> QGFSLAQYLQEQKTIVETALDQSLVITEPVTIYEAMRYSLLAGGKRLRPILCLAACEMLGGTAAMAMNTACALEMIHTMSLIHDDLPAMDNDDLRRGKPTNHKVYGEDIAILAGDALLSYAFEYVARTPDVPAERLLQVIVRLGQAVGAEGLVGGQVVDLESEGKDVAVETLNFIHTHKTGALLEVCVTAGAILAGAKPEEVQLLSRYAQNIGLAFQIVDDILDITVTYPKSQAEAQKLVAEAIASLEPYGEKANPLKALAEYI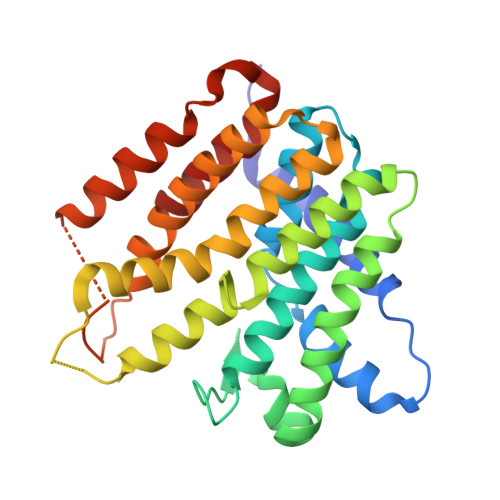VNA Here we report the biochemical and structural characteristics of Cfl1 and Cfl2, two Cif-like epoxide hydrolases from Burkholderia cenocepacia. EHs that belong to the α/β hydrolase superfamily of enzymes utilize an Asp-His-Asp/Glu catalytic triad to open the epoxide ring substrate and release the vicinal diol product. Cfl1 and Cfl2 also appear to utilize a Cif-like His-Tyr epoxide ring-opening pair instead of the classical Tyr-Tyr pair. While Cif and aCif exist as constitutive dimers, our hydrodynamic and structural studies revealed that Cfl1 and Cfl2 exist as octamers and decamers, respectively, by forming rings of dimers.

In contrast, Cfl2 shows very low activity against a diverse set of epoxides. The H-G-W-P sequence of Cfl1 follows the canonical H-G-X-P motif, whereas Cfl2 substitutes the histidine with an alanine (A-G-F-P). Each assembly is formed by a ring of dimers: a tetrameric ring of dimers in the case of Cfl1, and a pentameric ring in the case of Cfl2. In Cif, the equivalent residue His128 does not form a hydrogen bond with the catalytic water. In contrast to Cfl1, the catalytic side chains of Cfl2 show a much more similar alignment those of Cif (inset). The most striking difference is in the canonical dimer (1:2) interface, which is 1080 ​Å2 larger in Cfl2 than in Cfl1 and has a substantially more favorable predicted binding energy. Given this striking difference, we also analyzed the corresponding Cif and aCif dimer interfaces. We found that the surface area of the canonical dimer interface of Cfl2 is very similar to those of Cif and aCif, albeit with a modestly higher contribution from hydrophobic residues; the Cfl1 dimer interface is markedly smaller than all of the others. Similarly, in Cfl2, the N-terminus of monomer 1 makes several electrostatic interactions with monomer 3 and a hydrophobic interaction between Pro17 and Tyr287 (cluster 1). As a result, within the Cfl1 ring, the three dominant modes include interdimer flexion, seen in the form of new areas of deformation which correspond to its oligomer interfaces that are lacking from the ex circulum Cfl1 dimer (bottom row). This is not the case with Cfl2, where the ex circulum dimer loses its deformability at the dimer interface once it oligomerizes but the oligomer interface deformations do not compensate to the same degree as they do in Cfl1 (bottom row). The lack of substantial Cfl2 activity raises the possibility that it may function as a non-catalytic pseudoenzyme in vivo. However, this is not the case with Cfl2, which maintains the epoxide hydrolase motifs in its amino acid sequence and 3-dimensional arrangement of its catalytic residues.

>[10x]MYQHQSTEAASHLEATPYFREDPRLTGFRHRFDTVDGVRLHFVEGGRADGETIVLLAGFPESWYAWRRVMPLLADEFRIVAPDLPGQGDSDRPLVGYDTQTVAATLARLLERQNIARFYLAAHDVGAWVAYPFAAMYPESVKRLALLDAGIPGVTLPAALPIEPGNAWRTWHFAFHTVADLPETLIAGKEREYLDWFLRRKAANPESFSDADVDEYLRVFTRDGGLRAGLAFYRAVSESSAQNRKLQALGKLKMPVLAVSADQGSIPDMAGPLEHVAEEVTAATIAYSGHFIPEEQPQALARELRDFFR>[10x]GSHMKHTELRAAVLDALEKHDTGATFFDGRPAVFDEADFPAVAVYLTGAEYTGEELDSDT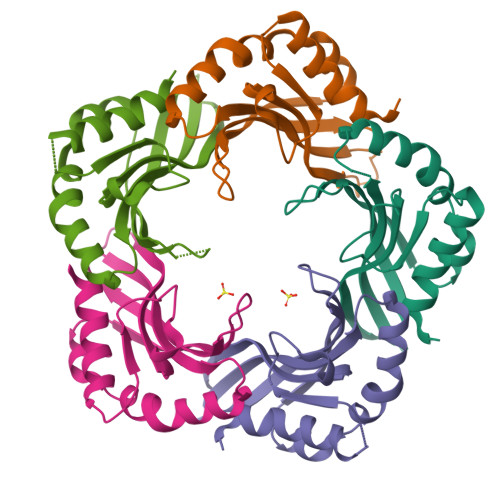WQAELHIEVFLPAQVPDSELDAWMESRIYPVMSDIPALSDLITSMVASGYDYRRDDDAGLWSSADLTYVITYEM> GEKTYVKRLVKILLLGAGESGKSTFLKQMRIIHGQDFDQRAREEFRPTIYSNVIKGMRVLVDAREKLHIPWGDNKNQLHGDKLMAFDTRAPMAAQGMVE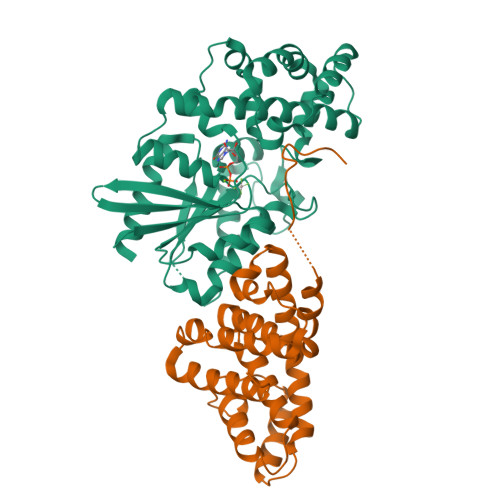TRVFLQYLPAIRALWEDSGIQNAYDRRREFQLGESVKYFLDNLDKLGVPDYIPSQQDILLARRPTKGIHEYDFEIKNVPFKMVDVGGQRSERKRWFECFDSVTSILFLVSSSEFDQVLMEDRQTNRLTESLNIFETIVNNRVFSNVSIILFLNKTDLLEEKVQVVSIKDYFLEFEGDPHCLRDVQKFLVECFRGKRRDQQQRPLYHHFTTAINTENIRLVFRDVKDTILHDNLKQLMLQ;> GLIIGPEEDYDPGYFNNESDIIFQDLEKLKSHPAYLVVFLRYILSQADPGPLLFYLCSEVYQQTNPKDSRSLGKDIWNIFLEKNAPLRVKIPEMLQAEIDLRLRNNEDPRNVLCEAQEAVMLEIQEQINDYRSKRTLGLGSLYGENDLLGLDGDPLRERQMAEKQLAALGDILSKYEEDRSAPMDFAVNTFMSHAGIRLRESR> MAIYADNSYSIGNTPLVRLKHFGHNGNVVVKIEGRNPSYSVKCRIGANMVWQAEKDGTLTKGKEIVDATSGNTGIALAYVAAARGYKLTLTMPETMSLERKRLLCGLGVNLVLTEGAKGMKGAIAKAEEIVASDPSRYVMLKQFENPANPQIHRETTGPEIWKDTDGKVDVVVAGVGTGGSITGISRAIKLDFGKQITSVAVEPVESPVISQTLAGEEV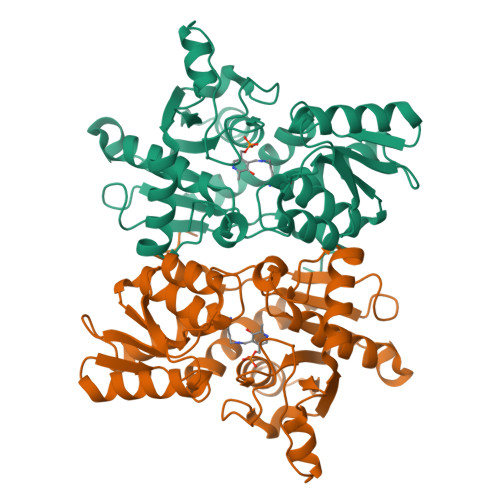KPGPHKIQGIGAGFIPKNLDLSIIDRVETVDSDTALATARRLMAEEGILAGISSGAAVAAADRLAKLPEFADKLIVVILPSASERYLSTALFEGIEG Central to the stringent response are the two unusual nucleotides ppGpp and pppGpp (collectively (p)ppGpp or alarmones). In contrast, short RSH-type alarmone synthetases only contain a synthetase domain and lack the hydrolase domain as well as regulatory domains found within the CTD of long RSH proteins. Members of this ‘small alarmone synthetase’ (SAS) family fall into the RelQ (also: SAS1) and RelP (also: SAS2) subclasses and are found in a wide range of bacteria including Bacillus subtilis, Staphylococcus aureus, Enterococcus faecalis and Listeria monocytogenes. In summary, RelP always appears as a highly active alarmone synthetase, while RelQ can switch between a passive state with low and an active (i.e. pppGpp-stimulated) state with high (p)ppGpp synthetase activity.

To better understand RelP at the molecular level, we determined the crystal structures of RelP homologues from S. aureus (Sa) and B. subtilis (Bs) at 2.25 and 3.3 Å resolution, respectively. Both, SaRelP and BsRelP form highly symmetrical and oval-shaped homotetramers with a prominent cleft in their centers highly reminiscent of BsRelQ. Helix α1 at the N-terminus of each monomer stabilizes the medial sides of the homotetramer interface via hydrogen bonds and salt bridges (buried surface area of ~1200 Å2). Helices α5 and α6 at the C-terminus of each monomer establish the lateral sides of the homotetramer interface mainly due to polar contacts (buried surface area of ~1200 Å2). The (p)ppGpp synthetase monomers of SaRelP and BsRelP are highly identical and consist of a mixed β-sheet build by five β-strands (β1–β5) that is surrounded by alpha helices (α1–α6). Structural comparison of RelP and RelQ reveals the architecture of the homotetramer as well as each of the monomers is highly similar (r.m.s.d. of 1.292 over 138 Cα atoms for the RelP and RelQ monomers). However, RelP and RelQ differ in the orientation of helix α2, which appears to be shifted approximately 3 Å towards the active site center in RelQ when compared to RelP. Another interesting observation is that the loop connecting β3 and β4, which is disordered in the structure of BsRelQ, could be resolved in both structures of RelP. In stark contrast, the G-Loop of SaRelP was well-ordered and could be unambiguously modeled in its apo- and ATP-bound structures.

>MGHHHHHHYVDRKPSLYLEDLRHDFKNSLSKFENGDEAFDTLLGFVELDHIYSSALKEISTKLSILDDNFNHIYKHNPIHHMERRVKEMRSLIEKLNRKGLQISAETAKEHILDIAGIRVVCNYLDDIYLIEEMLLKQEDVQLIKRKDYIQHPKENGYRSLHIVVSIPVFLAERVEVLPVEIQIRTIGMDMWASLEHKIRYKNNAETEKYRDLLKECATEITEVEDKLQQIHSEITE[2x]>MARGESGVLRVGFTASAAFNSVVPGAIRTFKRAYPDVRLQLEEGNTTQLADELNEGSLDVAFLRPGFTGNERFQLRLLSEEPMVIVLAETHPAAACKQIALSILKDEFFLLFPREIGLSLYDAVIKACGKAGFEPKIGQLVPQISSVINLVSAEMGVS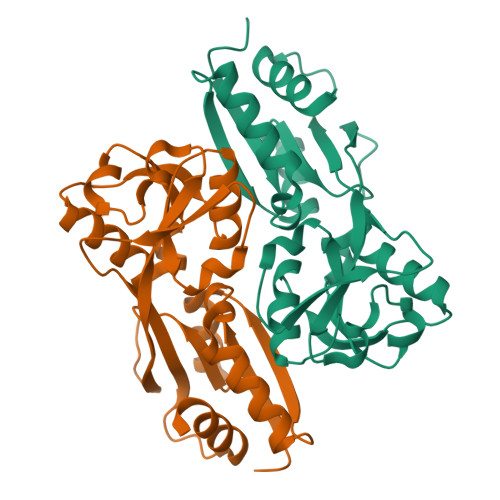MVPDSMRQVNVKGVVYRPVADQMPVAKLALAYRRGDTSPTLRNFILKVTG[4x]>MSGRLTGKVALVSG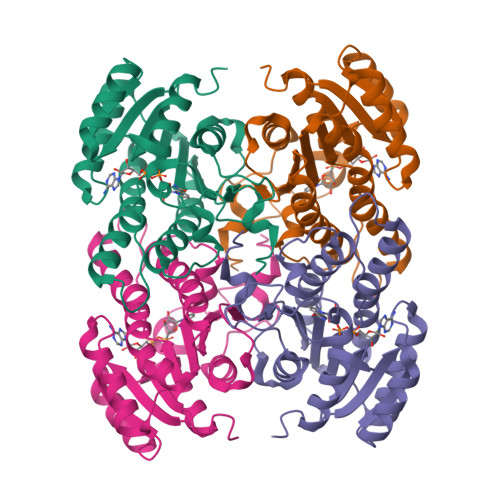GARGMGASHVRAMVAEGAKVVFGDILDEEGKAMAAELADAARYVHLDVTQPAQWKAAVDTAVTAFGGLHVLVNNAGILNIGTIEDYALTEWQRILDVNLTGVFLGIRAVVKPMKEAGRGSIINISSIEGLAGTVACHGYTATKFAVRGLTKSTALELGPSGIRVNSIHPGLVKTPMTDWVPEDIFQTALGRAAEPVEVSNLVVYLASDESSYSTGAEFVVDGGTVAGLAHNDFGAVEVSSQPEWVT[2x]>MNDKKIELLTTYLSLYIDHHTVLADMQNATGKYVVLDVRNAPAQVKKDQIKGAIAMPAKDLATRIGELDPAKTYVVYDWTGGTTLGKTALLVLLSAGFEAYELAGALEGWKGMQLPLE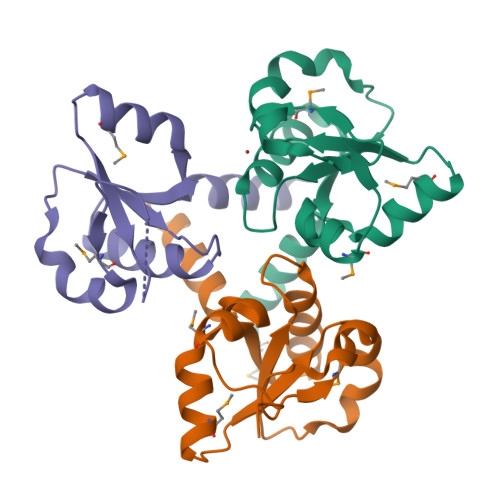HHHHHH[3x]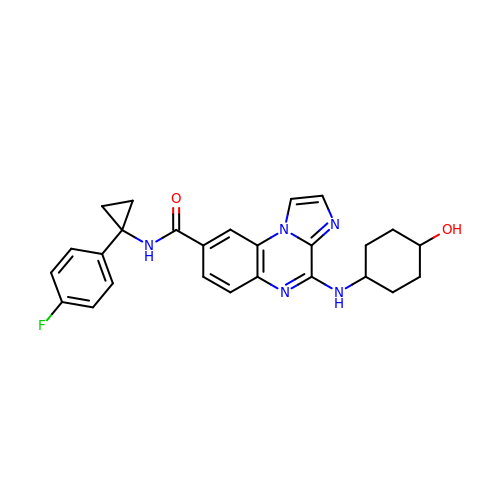N-[1-(4-fluorophenyl)cyclopropyl]-4-[(trans-4-hydroxycyclohexyl)amino]imidazo[1,2-a]quinoxaline-8-carboxamide | C26 H26 F N5 O2 | MFJOWCFANZXQBU-MXVIHJGJSA-N2-(4-methylpiperidin-1-yl)-N-[3-(propan-2-yl)-1,2-oxazol-5-yl]acetamide 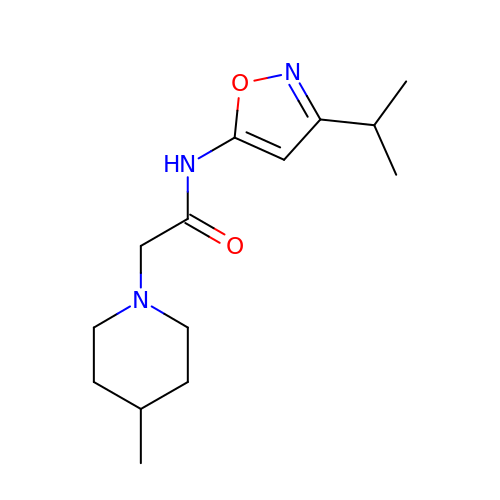| C14 H23 N3 O2 | RUCYUQYOHAXRGD-UHFFFAOYSA-N>MMVLVSYDVSTSSPGGDKRLRKVAKACRDLGQRVQ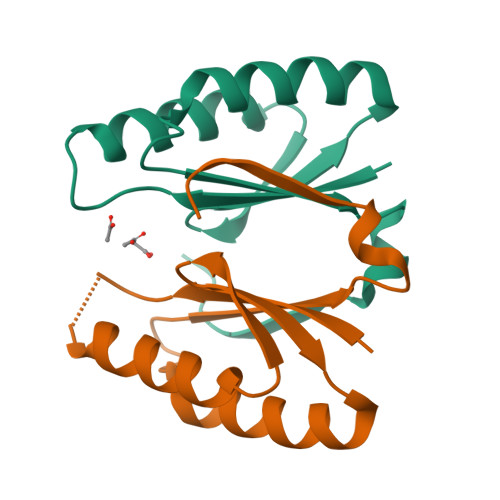FSVFEIEVDPAQWTALRQRLCDLIDPDIDSLRFYHLGAKWEARVEHVGAKPSLDLKGPLIFLEHHHHHH[2x]[(2R,3S,4R,5R)-5-(2,4-dioxo-3,4-dihydropyrimidin-1(2H)-yl)-3,4-dihydroxytetrahydrofuran-2-yl]methyl hydrogen (S)-{3-[(2R,3R,4R,5R,6R)-3,4,5-trihydroxy-6-(hydroxymethyl)tetrahydro-2H-pyran-2-yl]propyl}phosphonate 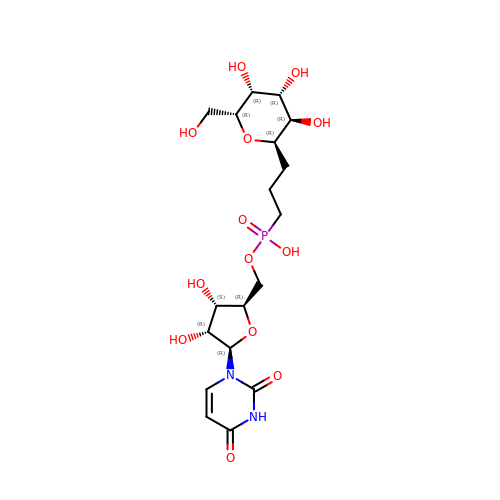| C18 H29 N2 O13 P | PDUJCKZVDKZKPQ-RUIRHDHUSA-N>MSTGDFLTKGIELVQKAIDLDTATQYEEAYTAYYNGLDYLMLALKYEKNPKSKDLIRAKFTEYLNRAEQLKKHLESEEANAAKKSPSAGSGSNGGNKKISQEEGEDNGGEDNKKLRGALSSAILSEKPNVKWEDVAGLEGAKEALKEAVILPVKFPHLFKGNRKPTSGILLYGPPGTGKSYLAKAVATEANSTFFSVSSSDLVSKWMGESEKLVKQLFAMARENKPSIIFIDEVDALTGTRGEGESEASRRIKTELLVQMNGVGNDSQGVLVLGATNIPWQLDSAIRRRFERRIYIPLPDLAARTTMFEINVGDTPCVLTKEDYRTLGAMTEGYSGSDIAVVVKDALMQPIRKIQSATHFKDVSTEDDETRKLTPCSPGDDGAIEMSWTDIEADELKEPDLTIKDFLKAIKSTRPTVNEDDLLKQEQFTRDFGQEGN[6x];>[12x]MASNAARVVATAKDFDKVGLGIIGYYLQLYAVELILSEEDRSQEMTALATELLDTIEAFKKEIGGESEAEDSDKSLHVMNTL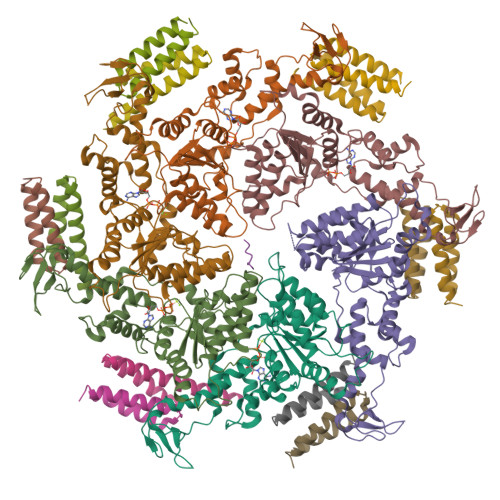IHDQEKAKIYMLNFTMSLYNEKLKQLKDGPWDVMLKRSLWCCIDLFSCILHLWKENISETSTNSLQKRIKYCKIYLSKLAKGEIGSSDEKTLDYADFADDSEEIKDEDVDHQTSDLENNNNDKVEGLAPKDQTTSYEPVDEVPEFIDDADSVNEEEQTVDKNEDAITKDEQQVVKKEVDLTRPSAPSEPAAAEHKSYTKDELTKIMDRASKIEQIQKLAKYAISALNYEDLPTAKDELTKALDLLNSI>MTNVLIVEDEQAIRRFLRTALEGDGMRVFEAETLQRGLLEAATRKPDLIILDLGLPDGDGIEFIRDLRQWSAVP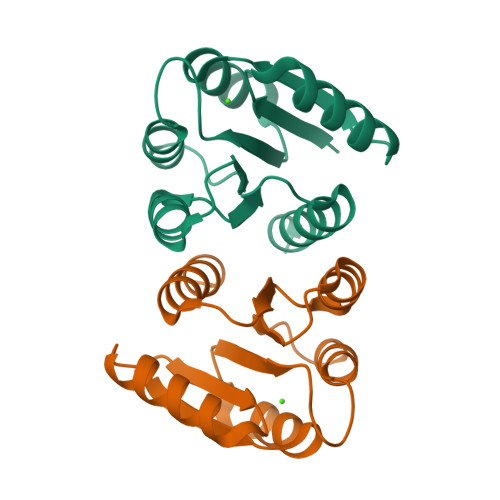VIVLSARSEESDKIAALDAGADDYLSKPFGIGELQARLRVALRRHSQ[2x]>SKNRISWVGDAVKTDGKKSYYKKVCIDSETLEVGDCVSVIPDDSSKPLYLARVTALWEDSSNGQMFH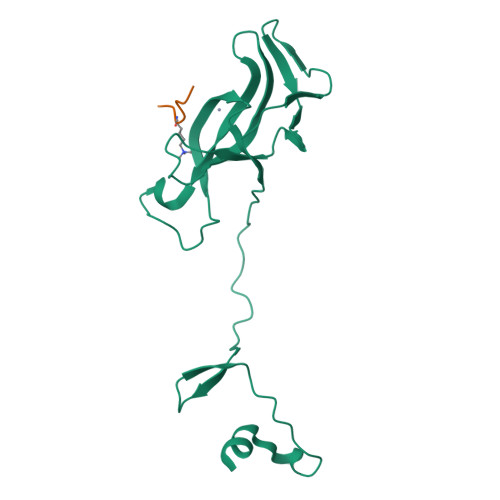AHWFCAGTDTVLGATSDPLELFLVDECEDMQLSYIHSKVQVIYKAPSGAGSATYFYQLWYDQDYARFESPPKTQPTEDNKYKFCASCARLA[4x];>GAKRHRKVLRDNY[4x]>MASHLASIYGTEQDKVNCSFYYKIGACRHGERCYRKHVKPNFSQTILCPNMYKNPIHEPNGKKFTQRELAEQFDAFYEDMFCEFSKYGEVEQLVVCDNVGDHLVGNVYVRFKYEESAQNAIDDLNSRWYSQRPVYAELSPVTDFREACCRQHETSECQRGGLCNFMHAKKPSPQLLRDLVLAQRKYLALNAAEEMKKEPNSDSTNRWVSVTAERKN[9x];>SSVGRSRSPPPSRERSVRSIEQELEQLRDVTPINQWKRKRSLWDIKPPGYELVTADQAKMSGVFPLPGA[9x]

On the other hand, U2AF small subunit, U2AF1, binds to the 3′ side of the boundary sequence between the exon and intron, known as the 3′ splice site (3′SS). Then, the recognition of 3′SS by U2AF1 is a critical step for the determination of the excluded intron for the production of mature mRNA. U2AF1 consists of conserved three domains, an N-terminal zinc finger (ZF1), a U2AF homology motif (UHM), and a C-terminal zinc finger (ZF2). As U2AF1 was stabilized by the binding of U2AF223, structural and biochemical experiments were carried out with a complex of Schizosaccharomyces pombe U2AF1 with the short fragment of U2AF2 spanning residues 93–161 (the U2AF1 complex), as previously reported.

One of the hot spot for such mutations is Ser34 in U2AF1; replacement of Ser34 with Tyr or Phe residues induces aberrant splicing. To elucidate further the impaired RNA recognition mechanism of the S34F/Y mutants, we attempted to crystallize the S34Y mutant with bound RNA (5′-UAGGU, 5′-AAGGU, or 5′-CAGGU). This mutant was chosen because its solubility is higher than that of S34F mutant, making it more likely to find suitable crystallization conditions. Although the 5′-AAGGU and 5′-CAGGU complexes did not crystallize, the crystal structure of the complex between the S34Y mutant and 5′-UAGGU was determined. In the complex, O4-carbonyl oxygen of −3U maintains a hydrogen bond with the amide proton of the mutated residue (Tyr34), despite a small but distinct position shift of the uridine base compared to that in wild-type U2AF1. Along with the imidazole ring of His29, the aromatic ring of Tyr34 also stacks against the −3U base, forming a π–π interaction that is absent from the wild-type complex. The S34Y and S34F mutants therefore bind 5′-UAAGGU with an affinity similar to that of wild-type protein for 5′-UUAGGU. In contrast to wild-type U2AF1, therefore, the S34Y and S34F mutants show little discrimination for the base at −3 position, except for rejecting guanosine. The S34F/Y mutations clearly allow much greater flexibility in the selection of splice sites with U, C, or A at the −3 position.N-(6-aminopyridin-3-yl)-5-hydroxy-1-phenylpyrazole-4-carboxamide | C15 H13 N5 O2 | 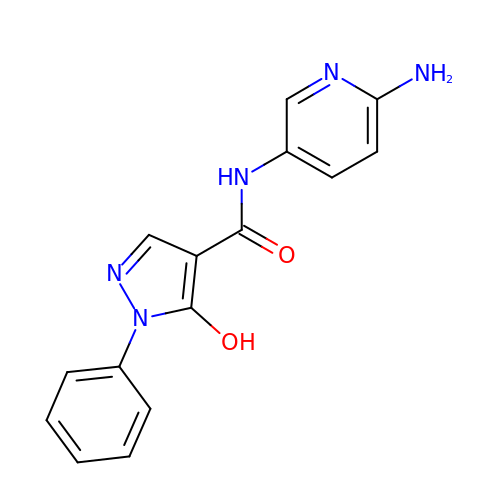XRMPIZHDSBHDCD-UHFFFAOYSA-N>[2x]XADEIAKAQVARPGGDTIFGKIIRKEIPAKIIFEDDRCLAFHDISPQAPTHFLVIPKKHISQISVAEDDDESLLGHLMIVGKKCAADLGLNKGYRMVVNEGS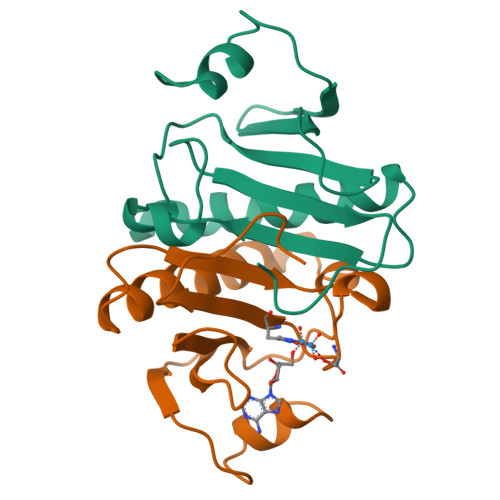DGGQSVYHVHLHVLGGRQMHWPPG> MAHHHHHHDYGIPTTENLYFQGSIENLPAFPREKLTLRLLLGSGAFGEVYEGTAVDILGVGSGEIKVAVKTLKKGSTDQEKIEFLKEAHLMSKFNHPNILKQLGVCLLNEPQYIILELMEGGDLLTYLRKARMATFYGPLLTLVDLVDLCVDI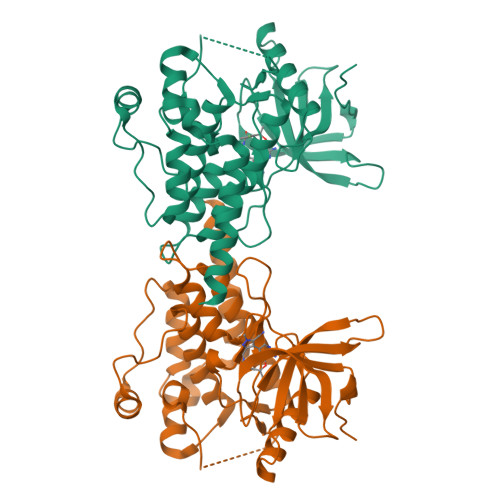SKGCVYLERMHFIHRDLAARNCLVSVKDYTSPRIVKIGDFGLARDIYKNDYYRKRGEGLLPVRWMAPESLMDGIFTTQSDVWSFGILIWEILTLGHQPYPAHSNLDVLNYVQTGGRLEPPRNCPDDLWNLMTQCWAQEPDQRPTFHRIQDQLQLFRNFFLNSIYKSRDE>[2x]AKDYTNEAIFTQFDVNPKGLINNPSQPIEFNLAFSDMNNGQKVKFKPGDFFDLTLPSNDEVSLRSLRAMGSKMPVLAKDKNGKEITLGELTFNGSHIHFEFMEDVLQLENVTGTINLKSVYDNAYRGEDDKIAELPTNLGLGSLDKQMITISQPGTPTGVEPSPIFYWKTGTFSTEVHGDMNWWLNIN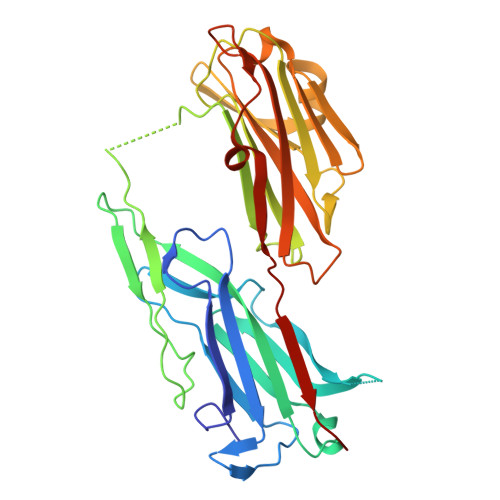SPKEAVQSDVKVIDTIGEGHKLVDGSIMVDVEANGELKHISAEAFNKEYGTITVEGQVLTVMIPKEKAAKTTFTVTYDTRAFDKKLENYKNSSTIEYKDESGNLVTDTPKHYTDTSVVNMFDDATIGGEMKDK> MATMQCDVVSVKESIYSGAVTMLIAKGAGGELGILPGHAPLVTLLQPGPIRVLLENGTEEIVYVSGGVLEVQPHVVTVLADTAIRADNLDEAAILEARK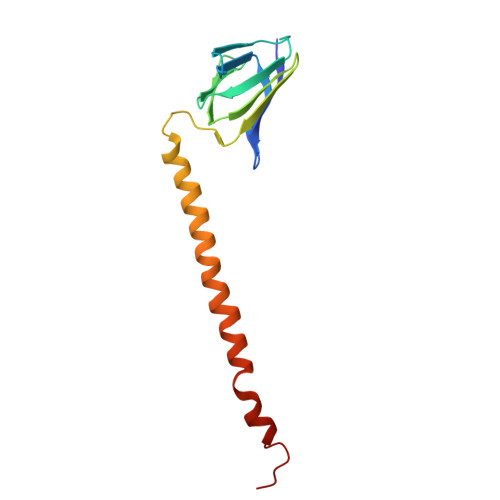NAEQLLANQKSDLDSAAALAALAETAAQLETIRKIKNRAQ>NSINDSKILSLQNKKNALVDTSGYNAEVRVGDNVQLNTIYTNDFKLSSSGDKIIVNLNNNILYSAIYENSSVSFWIKISKDLTNSHNEYTIINSIEQNSGWKLCIRNGNIEWILQDVNRKYKSLIFDYSESLSHTGYTNKWFFVTITNNIMGYMKLYINGELKQSQKIEDLDEVKLDKTIVFGIDENIDENQMLWIRDFNIFSKELSNEDINIVYEGQILRNVIKDYWGNPLKFDTEYYIINDNYIDRYIAPESNVLVLVQYPDRSKLYTGNPITIKSVSDKNPYSRILNGDNIILHMLYNSRKYMIIRDTDTIYATQG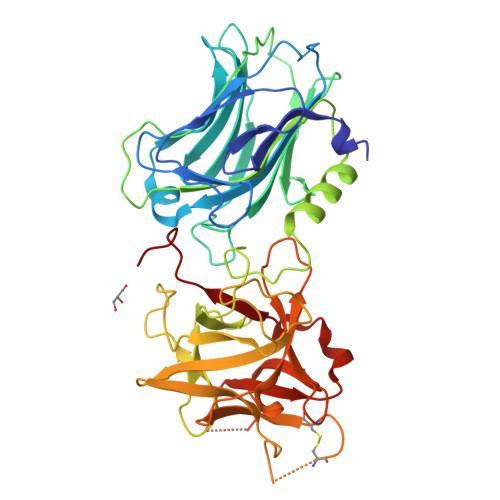GECSQNCVYALKLQSNLGNYGIGIFSIKNIVSKNKYCSQIFSSFRENTMLLADIYKPARFSFKNAYTPVAVTNYETKLLSTSSFWKFISRDPGWVE[4x]> MTNQQYGFQFQKKTTDGTDLSADQLKAMQFNLTQYSDNSFQQASKTNAITSTDLQALAPGYYGIQEAAAPTGYQLDGTTYLFQLTSDGQWQYHGTKD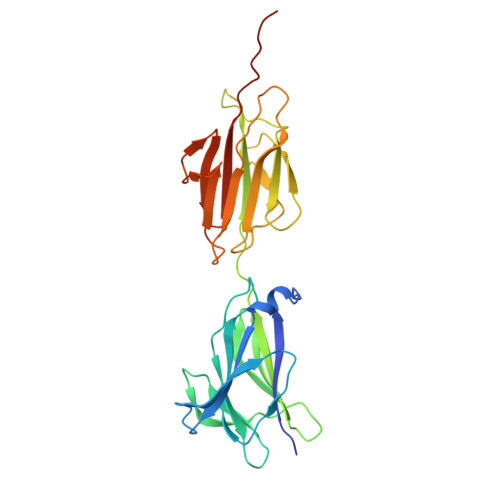NVTSGSVINGQQTLNPVGDKSDDFTVTGDHQQILTLTKYDEPKPSMTLRVIKQDNQSQYLAGAAFTLQPSAGEAETITSSATSEGQAFATKLVADGTYTMSETKAPDGYQSNPAKIAIQVATTGKEATVTIDGEALKPGESKNGYTLAIDGSTITLQAINQPLAILPLEHHHHHH> MEALGMIETRGLVALIEASDAMVKAARVKLVGVKQIGGGLCTAMVRGDVAACKAATDAGAAAAQRI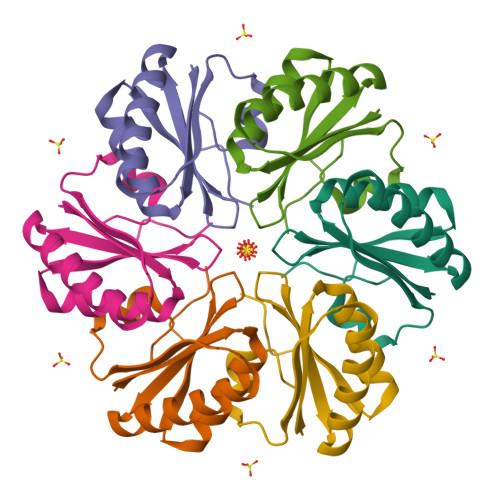GELVSVHVIPRPHGDLEEVFPIGLKGDSSNLHHHHHH>QTDMSRKAFVFPKESDTSYVSLKAPLTKPLKAFTVCLHFYTELSSTRGYSIFSYATKRQDNEILIFWSKDIGYSFTVGGSEILFEVPEVTVAPVHICTSWESASGIVEFWVDGKPRVRKSLKKGYTVGAEASIILGQEQDSFGGNFEGSQSLVGDIGNVNMWDFVLSPDEINTIYLGGPFSPNVLNWRALKYEVQGEVFTKPQLWP[10x]

C-reactive protein (CRP) is a pentameric protein of 115 kDa composed of five identical non-covalently associated pentraxin domains. The B-face binds to a range of ligands, with the canonical example being phosphocholine (PCh) head groups in lipids such as phosphatidylcholine. This is a calcium-dependent interaction, with each CRP monomer chelating two adjacent Ca2+ ions. The A-face modulates many effector functions of CRP, such as activation of the classical complement pathway, where binding of complement component C1q to CRP is mediated via predominantly electrostatic interactions between the Ca2+-containing globular head domain of C1q (gC1q) and the A-face of CRP.

Decameric CRP is formed from the offset stacking of two pentamers via their A-faces. Intermolecular contacts between monomers within CRP decamers were also dominated by non-covalent ionic bonds, which formed a second ionic zipper, perpendicular to that found in CRP pentamers. Ionic bonds included Asp163(chain A)–Arg188(J), Glu170(A)–Arg6(J), Arg188(E)–Asp163(F), Arg188(B)–Asp169(H) and Asn172(C)–Ser181(G). Asp169 and Arg6 were able to form additional salt bridges in decamers compared to those formed in pentamers, whilst still participating in monomer-monomer interactions. Although decamers appeared to adopt C2 symmetry, they were solved without symmetry applied and reached resolutions of 3.3 – 2.8 Å. No major differences were observed between the decamers at different pHs, with or without PCh, other than the proportions of decamers to pentamers. Intermonomeric ionic bonds found in decameric CRP at both pH 7.5 and pH 5 were similar to the crystal structures and the cryoEM-derived pentameric CRP at pH 7.5, except for at Glu197-Lys123 where there was a larger distribution of bond lengths, indicating conformational flexibility at this location. The proportions of these varied between conditions, with pH 5 containing more decamers than at pH 7.5, 68% vs 44% decamers, respectively. No crystallization is required for cryoEM using single-particle analysis, hence these decamers represent solution-phase structures of CRP, previously posited based on analytical ultracentrifugation (AUC). Residues implicated in C1 binding and/or complement activation are predominantly located on the A-face, and therefore binding of C1q to CRP will be sterically hindered by decamerization, which could inhibit complement activation by CRP at low pH.> GGSGNEPTQEKHFMVYYRAWRDKTMQGVNTTLPDENWLTMHDIPYGIDIVNVFSYVPKGQEALAQPFYDTLKNEYAPALHARGVRLVRGIDYSELLKVPYAGTTPTEAEFDAYAKELLTKFVDDLGIDGLDIDMETRPSEKDIVLSNGVIRALSKYIGPKSGTDRPFLYDTNAEYLPPLQDVSDCFDFLAYQQYG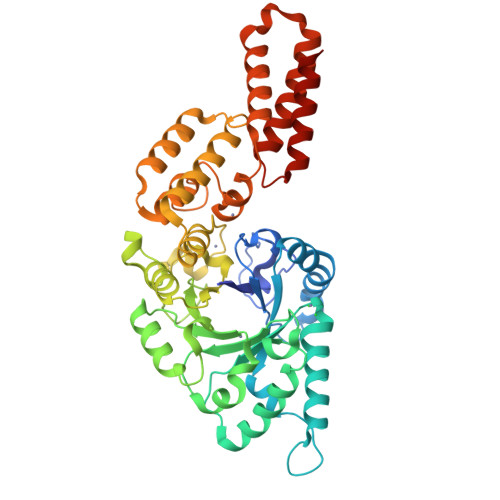SDDKRTQRALNNLSPVLNGERFVPGLTFPEEQDRNRWYDTKEPYMESNMYKVARYSYENNLGGMFLYALDRDGRTYNEDDLNQIKPSNLLWTKTAIAESKGVSLAEMKAAAQHYLKRISYANTDLEAQNKAAETVTQATTLYDVNKAILGGDYGQGLSNTYDAELEKGLLAIDLTTLYRALDQAVAAIEKAESYTPETIQALQTTKESVATELAGKTYTAAQVTTWQTEVQTALDNLKEK>[4x]MHHHHHHHHENLYFQGSSSQEKNGKGEVIIPKEKFWKISTPPEAYWNREQEKLNRQYNPILSMLTNQTGEAGRLSNISHLNYCEPDLRVTSVVTGFNNLPDRFKDFLLYLRCRNYSLLIDQPDKCAKKPFLLLAIKSLTPHFARRQAIRESWGQESNAGNQTVVRVFLLGQTPPEDNHPDLSDMLKFESEKHQDILMWNYRDTFFNLSLKEVLFLRWVSTSCPDTEFVFKGDDDVFVNTHHILNYLNSLSKTKAKDLFIGDVIHNAGPHRDKKLKYYIPEVVYSGLYPPYAGGGGFLYSGHLALRLYHITDQVHLYPIDDVYTGMCLQKLGLVPEKHKGFRTFDIEEKNKNNICSYVDLMLVHSRKPQEMIDIWSQLQSAHLKC

β1,3-N-acetylglucosaminyltransferases (B3GNTs) are Golgi-resident glycosyltransferases involved in the biosynthesis of poly-N-acetyl-lactosamine chains. They catalyze the addition of the N-acetylglucosamine to the N-acetyl-lactosamine repeat as a key step of the chain elongation process. Among the characterized B3GNTs, B3GNT2 is the major poly-N-acetyl-lactosamine synthase, and deletion of its coding gene dramatically reduced the cell surface poly-N-acetyl-lactosamine and led to hypersensitive and hyperresponsive immunocytes. The luminal domain of B3GNT2 comprises an N-terminal helical domain (Pro55–Cys125) and a C-terminal catalytic domain (Cys138–Cys397) as well as an extended linker (Arg126–Lys137) that connects the helical domain to the catalytic domain.

The luminal domain structure of B3GNT2 was solved by single-wavelength anomalous dispersion phasing using an iodide derivative to a resolution of 2.50 Å. Subsequently, B3GNT2 structures in apo form or in complex with either substrates or products were determined by molecular replacement using the iodide derivative structure as the template. The six structures presented here were solved in different space groups and the number of molecules in the asymmetric unit also varied. The recombinant proteins used for crystallization contain residues Ser31–Cys397 or Lys45–Cys397, but only residues Pro55–Cys397 are well defined in the electron density maps, except for a disordered loop between residues Leu77 and Ser88.>[4x]MGSKFIQNAAEIA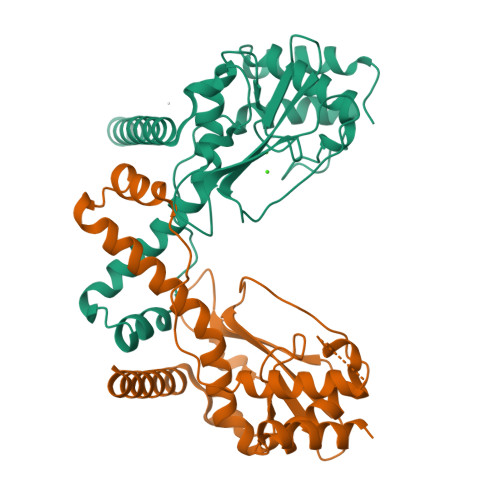KKAMDSVDPSLSEKFTIVIRFLTDNPDAASALKGKERSIVGTEEYIIASATNFKKGRDPRTPLPPSTIPDEMVSVILNKYFEVPSEELEKAEEWHRLSMGAENIVGDLLERYIAEVIEPHGWIWCSGSMVRAVDFIYCDSENVWQSLQVKNRDNTENSSSAAIRHGTPIKKWFRTFSKKRGDNWDKFPSLEGKENLSEKGFKLYVEKYLSALRAIKALEHHHHHH(2R,3S,4R,5R,6R)-2,6-difluoro-2-(hydroxymethyl)tetrahydro-2H-pyran-3,4,5-triol | 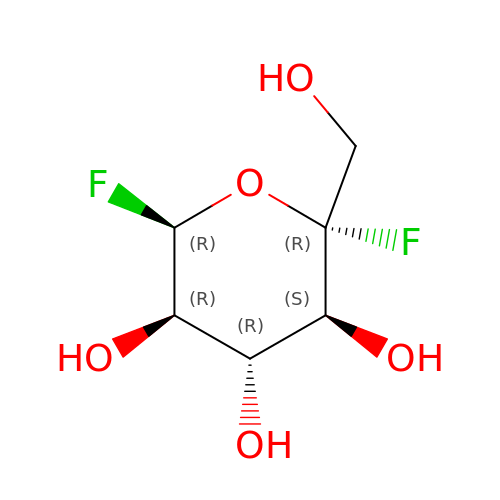C6 H10 F2 O5 | MGHYRMVVRYCAON-PQMKYFCFSA-N> GAHMDCHLSDMLQQLHSVNASKPSERGLVRQEEAEDPACIPIFWVSKWVDYSDKYGLGYQLCDNSVGVLFNDSTRLILYNDGDSLQYIERDGTESYLTVSSHPNSLMKKITLLKYFRNYMS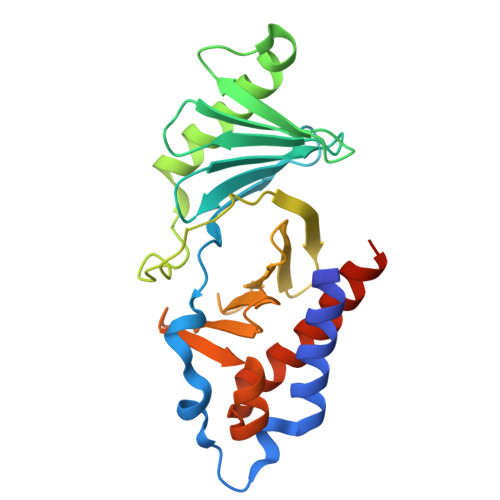EHLLKAGANITPREGDELARLPYLRTWFRTRSAIILHLSNGSVQINFFQDHTKLILCPLMAAVTYIDEKRDFRTYRLSLLEEYGCCKELASRLRYARTMVDKLLSSRSASNRLKAS> MSPAKDVKVYKKILDQNKDIQDLLDKIVFDAQHGQIWFDENRMLLMHTSILGFLRKDLYQMLGLERTKRFFIRCGYQAGMRDAEVTSKLRPNLNEAEAFMAGPQMHGIRGMVQVEVNELHLSHDLKQFYADFNWLNSFEAEVHLSEFPASDQPACWMLLGYACGYSSFVMGQTIIY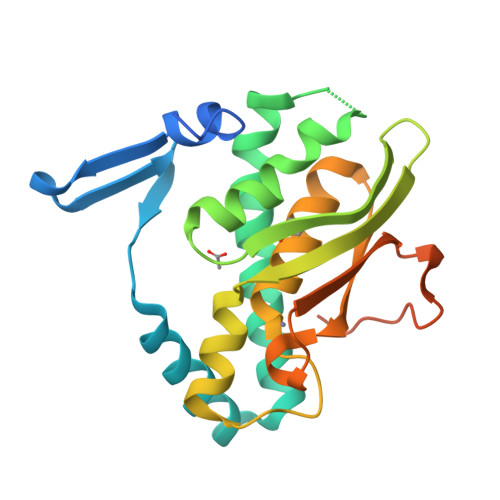QETHCVAQGDEHCRIIGKPLSEWENADELIRFMSPDAVSDEIIALQAELNQLK>[2x]TATDNARQVTIIGAGLAGTLVARLLARNGWQVNLFERRPDPRIETGARGRSINLALAERGAHALRLAGLEREVLAEAVMMRGRMVHVPGTPPNLQPYGRDDSEVIWSINRDRLNRILLDGAEAAGASIHFNLGLDSVDFARQRLTLSNVSGERLEKRFHLLIGADGCNSAVRQAMASVVDLGEHLETQPHGYKELQITPEASAQFNLEPNALHIWPHGDYMCIALPNLDRSFTVTLFLHHQSPAAQPASPSFAQLVDGHAARRFFQRQFPDLSPMLDSLEQDFEHHPTGKLATLRLTTWHVGGQAVLLGDAAHPMVPFHGQGMNCALEDAVALAEHLQSAADNASALAAFTAQRQPDALAIQAMALENYVEMSSKVASPTYLLERELGQIMAQRQPTRFIPRYSMVTFSRLPYAQAMARGQIQEQLLKFAVANHSDLTSINLDAVEHEVTRCLPPLSHLS

Kynurenine 3-monooxygenase (KMO) regulates levels of neuroactive kynurenine pathway metabolites associated with neurodegeneration. Downregulation of KMO activity shifts the flux between the two branches of the KP toward increased KYNA formation, thus generating a neuroprotective environment. The KMO reaction is a random bi–bi mechanism proceeding through a ternary complex of KMO-bound to l-KYN and NADPH (steady-state enzymatic assays are described in Supplementary Methods) with a turnover value, kcat, of 8.2 ± 0.2 s−1 and Km values for NADPH and l-KYN of 16.9 ± 1.5 and 12.1 ± 1.4 µM, respectively. We next determined crystal structures of KMO in complex with the novel inhibitors or with l-KYN to inform the design of small-molecule inhibitors capable of penetrating the blood–brain barrier.

Additional hydrogen bonding interactions are observed between the l-KYN carboxylate group and both Arg83 and Tyr97, as a direct consequence of the reorientation of both residues. Although the l-KYN aromatic moiety is located adjacent to the flavin isoalloxazine ring as previously reported, an additional water molecule is present that is located directly above the flavin C4a/N5. This is accompanied by a slight tilting of the flavin isoalloxazine. The position of the flavin isoalloxazine appears to be linked to the water molecule above C4a/N5 which, together with the adjacent water molecule located above the C10 atom, is likely to mimic the position of individual oxygen atoms in the proposed C4a peroxoflavin adduct. This suggests nucleophilic attack by the l-KYN occurs on the proximal oxygen, to generate a transient 3-oxo-l-KYN flavin adduct. Notably, l-KYN is known to stimulate KMO reduction by NADPH and other reported KMO inhibitors mimic this effect.> GHMLRRKFLRRDHRENIIRIFQEMADLNNALGEKYKVSSYHRSIESLKTNLDKPLNTPQDLKAFSGFGAKLLKKAEEIMATGKLEELESKTKPKLKAIQELTQVHGFGPRAAAALFDREGIFTVDELLQKADSIPSLTDQQRVGIKYFYDIN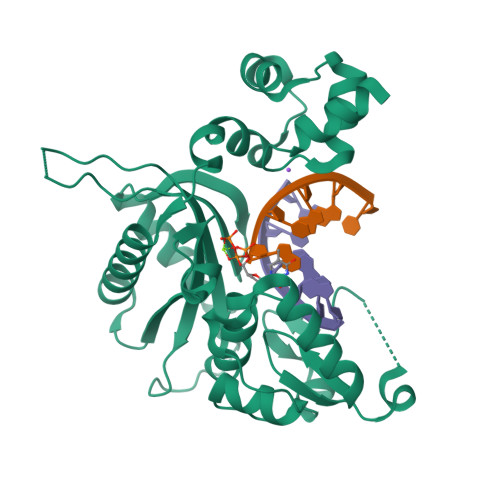EKIPMQESVLHENYLREKCMEVLGKDFSILICGSYRRRHPFSGDVDAILSRTLDAPPLSEPVAATGVLGHFVEFLESLKYLEATMAQGPLKYMGMGRLPPRIVRDKAGRENTKVYKARRVDIRLIETKSVPTAMLTFTGSKNFNVIMRQAAISKGYLLNEYGLFKLGTPEEARALYERIGIRGKNAGEELGVPKDELEDKRVEVRSEQDVFDVLGMPYAKPENRDP(2S)-2-[[(3S)-3-azanyl-4-oxidanyl-4-oxidanylidene-butanoyl]amino]-4-methyl-pentanoic acid | C10 H18 N2 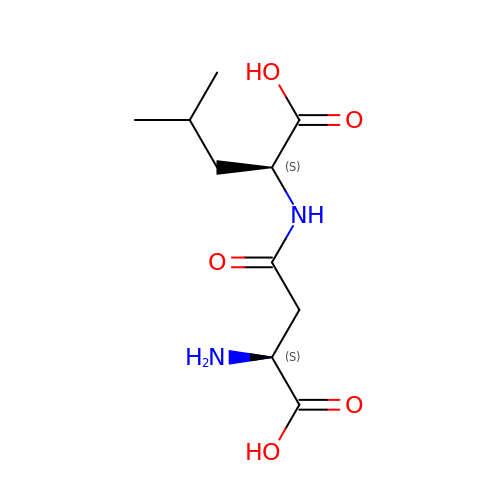O5 | IYJILWQAFPUBHP-BQBZGAKWSA-N>[2x]MREKPKYLPPTLRDKNRYIAFQVIGERPFKKDEIKKAVWEASLSALGYLGSARAKPWFIKFDEKSQTGIVRVDRKHVEELRFALTMLTEINGSKVIFRTLGVSGTIKRLKRKFLAEYGWR;>MSEEEVSFSRDYFVEMDVRDEEAHELASDWFDEVVFTKKLVLEDPPDWGSLKEELKELRGKYGKVALLLVTRKPSLIREVKSRNLKALLYVQGGDMRINR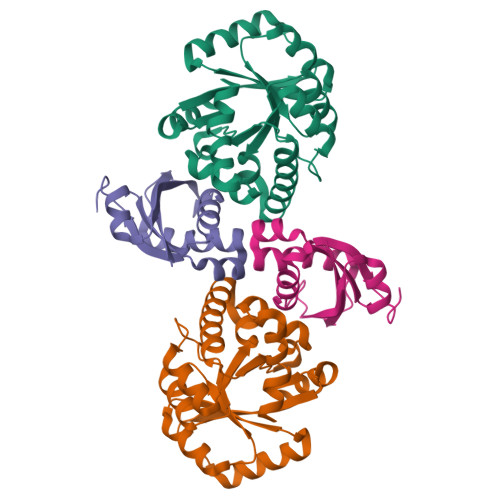MAIESGVDALISPWFGRKDPGFDHTLAGMAARRGVAIGFSLSPLLNANPYGRAQILRFMMKTWQLVKKYRVPRFITSSAESRWEVRGPRDLMSLGINIGMEIPEARASLNFYPRTIVWKL[2x]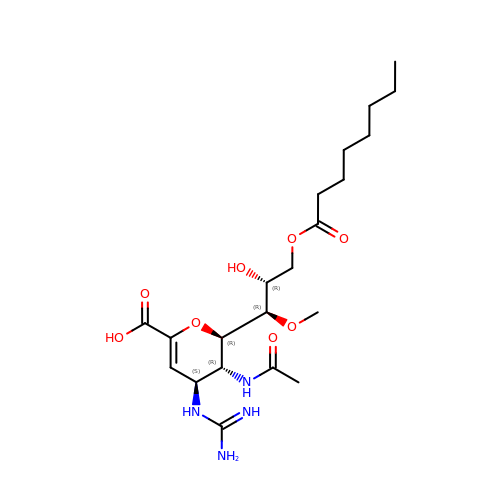5-acetamido-2,6-anhydro-4-carbamimidamido-3,4,5-trideoxy-7-O-methyl-9-O-octanoyl-D-glycero-D-galacto-non-2-enonic acid | C21 H36 N4 O8 | UKTIJASCFRNWCB-RMIBSVFLSA-N N-(carboxycarbonyl)-beta-D-glucopyranosylamine | C8 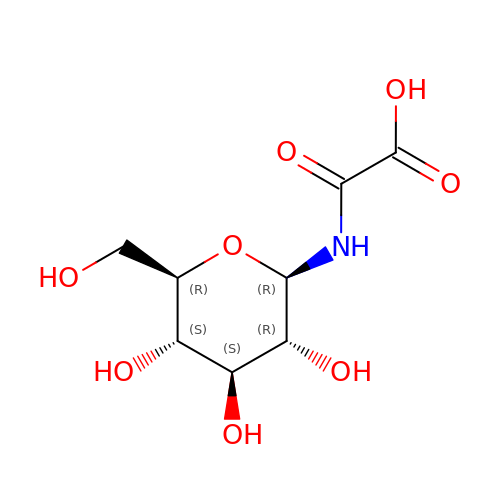H13 N O8 | ZSURXDJFFBVRAT-UHKLXPPTSA-N> MAEAGLRGWLLWALLLRLAQSEPYTTIHQPGYCAFYDECGKNPELSGSLMTLSNVSCLSNTPARKITGDHLILLQKICPRLYTGPNTQACCSAKQLVSLEASLSITKALLTRCPACSDNFVNLHCHNTCSPNQSLFINVTRVAQLGAGQLPAVVAYEAFYQHSFAEQSYDSCSRVRVPAAATLAVGTMCGVYGSALCNAQRWLNFQGDTGNGLAPLDITFHLLEPGQAVGSGIQPLNEGVARCNESQGDDVATCSCQDCAASCPAIARPQALDSTFYLGQMPGSLVLIIILCSVFAVVTILLVGFRVAPARDKSKMVDPKKGTSLSDKLSFSTHTLLGQFFQGWGTWVASWPLTILVLSVIPVVALAAGLVFTELTTDPVELWSAPNSQARSEKAFHDQHFGPFFRTNQVILTAPNRSSYRYDSLLLGPKNFSGILDLDLLLELLELQERLRHLQVWSPEAQRNISLQDICYAPLNPDNTSLYDCCINSLLQYFQNNRTLLLLTANQTLMGQTSQVDWKDHFLYCANAPLTFKDGTALALSCMADYGAPVFPFLAIGGYKGKDYSEAEALIMTFSLNNYPAGDPRLAQAKLWEEAFLEEMRAFQRRMAGMFQVTFMAERSLEDEINRTTAEDLPIFATSYIVIFLYISLALGSYSSWSRVMVDSKATLGLGGVAVVLGAVMAAMGFFSYLGIRSSLVILQVVPFLVLSVGADNIFIFVLEYQRLPRRPGEPREVHIGRALGRVAPSMLLCSLSEAICFFLGALTPMPAVRTFALTSGLAVILDFLLQMSAFVALLSLDSKRQEASRLDVCCCVKPQELPPPGQGEGLLLGFFQKAYAPFLLHWITRGVVLLLFLALFGVSLYSMCHISVGLDQELALPKDSYLLDYFLFLNRYFEVGAPVYFVTTLGYNFSSEAGMNAICSSAGCNNFSFTQKIQYATEFPEQSYLAIPASSWVDDFIDWLTPSSCCRLYISGPNKDKFCPSTVNSLN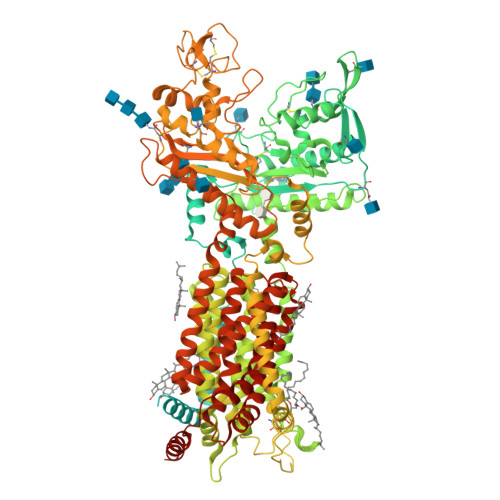CLKNCMSITMGSVRPSVEQFHKYLPWFLNDRPNIKCPKGGLAAYSTSVNLTSDGQVLASRFMAYHKPLKNSQDYTEALRAARELAANITADLRKVPGTDPAFEVFPYTITNVFYEQYLTILPEGLFMLSLCLVPTFAVSCLLLGLDLRSGLLNLLSIVMILVDTVGFMALWGISYNAVSLINLVSAVGMSVEFVSHITRSFAISTKPTWLERAKEATISMGSAVFAGVAMTNLPGILVLGLAKAQLIQIFFFRLNLLITLLGLLHGLVFLPVILSYVGPDVNPALALEQKRAEEAVAAVM>[4x]MCTSIIFSP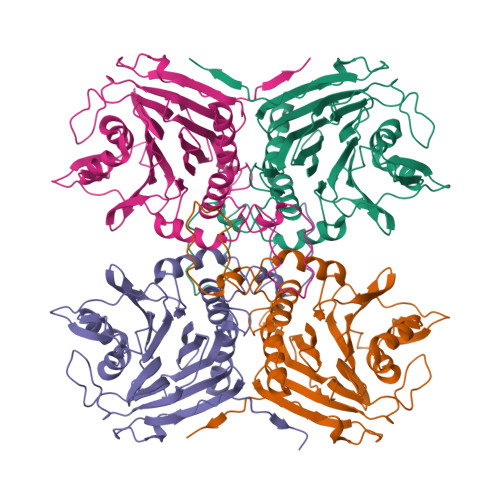KDHYFGRNLDLEITFGQQVVITPRNYTFKFRKMPSLKKHYAMIGISLDMDDYPLYFDATNEKGLGMAGLNYPGNATYYEEKENKDNIASFEFIPWILGQCSTISEVKDLLSRINIADLNFSEKMQASSLHWLIADKTGTSLVVETDKDGMHIYDNPVGCLTNNPQFPKQLFNLNNYADVSPKMPKNNFSDKVNMAGYSRGLGSHNLPGGMDSESRFVRVAFNKFNAPIAETEEENIDTYFHILHSVEQQKGLDEVGPNSFEYTIYSDGTNLDKGIFYYTTYSNKQINVVDMNKEDLDSSNLITYDMLDKTKFNHQNHHHHHH Caylin-1 | C30 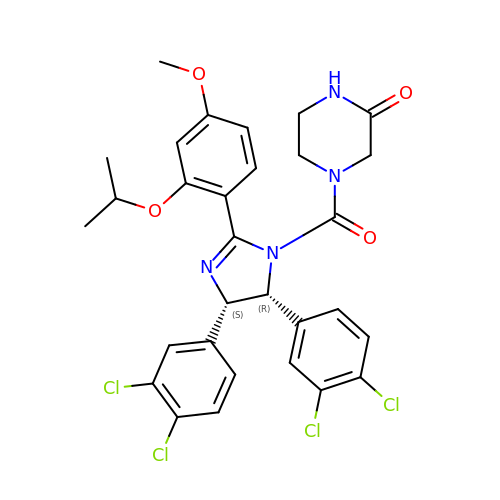H28 Cl4 N4 O4 | SOQGENPVVRSGAY-WUFINQPMSA-N>SLALHKVIMVGSGGVGKSALTLQFMYDEFVEDYEPTKADSYRKKVVLDGEEVQIDILDTAGQEDYAAIRDNYFRSGEGFLCVFSITEMESFAATADFREQILRVKEDENVPFLLVGNKSDLEDKRQVSV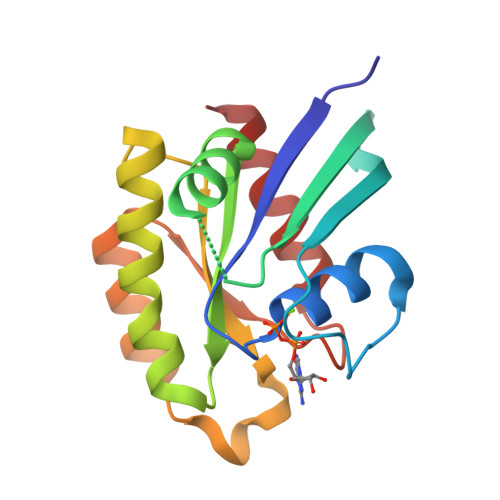EEAKNRADQWNVNYVETSAKTRANVDKVFFDLMREIRAR[2x]>CCAGCGCT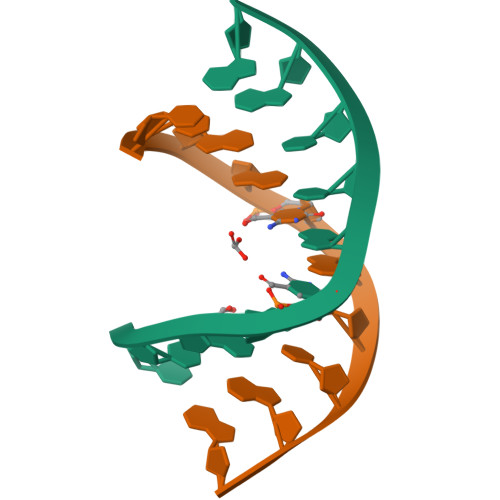GG[2x]>GDRVADVIESSIGDSVSRALTHALPAPTGQNTQVSSHRLDTGKVPALQAAEIGASSNASDESMIETRCVLNSHSTAETTLDSFFSRAGLVGEIDLPLEGTTNPNGYANWDIDITGYAQMRRKVELFTYMRFDAEFTFVACTPTGEVVPQLLQYMFVPPGAPKPDSRESLAWQTATNPSVFVKLSDPPAQVSVPFMSPASAYQWFYDGYPTFGEHKQEKDLEYGACPNNMMGTFSVRTVGTSKSKYPLVVRIYMRMKHVRAWIPRPMRNQNYLFKANPNYAGNSIKPTGASRTAITTL[5x];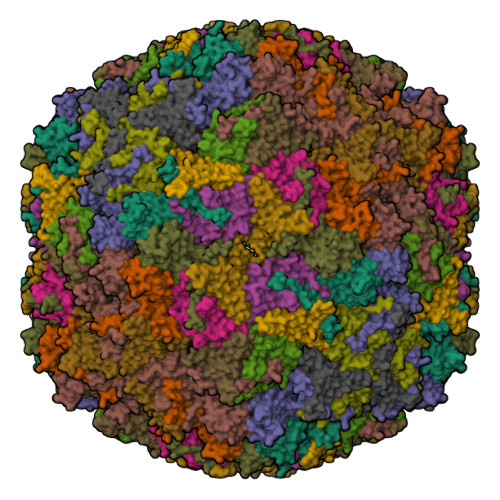>GFPTELKPGTNQFLTTDDGVSAPILPNFHPTPCIHIPGEVRNLLELCQVETILEVNNVPTNATSLMERLRFPVSAQAGKGELCAVFRADPGRSGPWQSTLLGQLCGYYTQWSGSLEVTFMFTGSFMATGKMLIAYTPPGGPLPKDRATAMLGTHVIWDFGLQSSVTLVIPWISNTHYRAHARDGVFDYYTTGLVSIWYQTNYVVPIGAPNTAYIIALAAAQKNFTMQLCKDASDILQTGTIQ[5x];>[5x]MGSQVSTQRSGSHENSNSATEGSTINYTTINYYKDSYAATAGKQSLKQDPDKFANPVKDIFTEMAAPLKSPSAEACGYSDRVAQLTIGNSTITTQEAANIIVGYGEWPSYCSDSDATAVDKPTRPDVSVNRFYTLDTKLWEKSSKGWYWKFPDVLTETGVFGQNAQFHYLYRSGFCIHVQCNASKFHQGALLVAVLPEYVIGTVAGGTGTEDSHPPYKQTQPGADGFELQHPYVLDAGIPISQLTVCPHQWINLRTNNCATIIVPYINALPFDSALNHCNFGLLVVPISPLDYDQGATPVIPITITLAPMCSEFAGLRQAVTQ>[2x]GAMDPFDASKVKCSGPGLERATAGEVGQFQVDCSSAGSAELTIEICSEA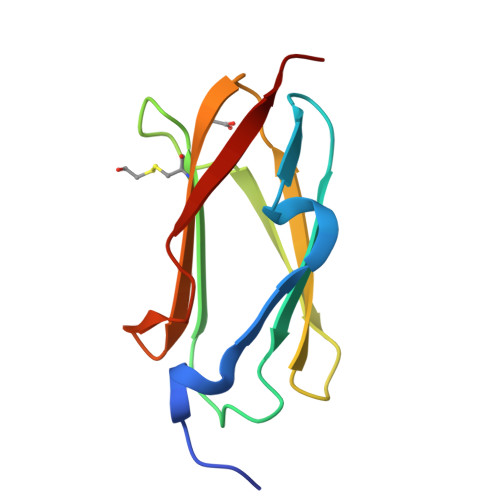GLPAEVYIQDHGDGTHTITYIPLCPGAYTVTIKYGGQPVPNFPSKLQVEPA>FACKTANGTAIPIGGGSANVYVNLAPVVNVGQNLVVDLSTQIFCHNDYPETITDYVTLQRGSAYGGVLSNFSGTVKYSGSSYPFPTTSETPRVVYNSRTDKPWPVALYLTPVSSAGGVAIKAGSLIAVLILRQ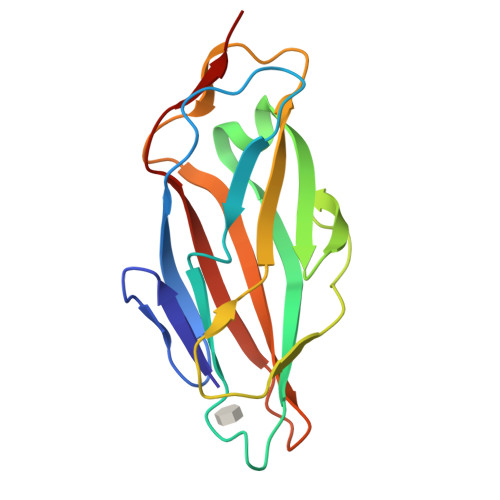TNNYNSDDFQFVWNIYANNDVVVPT[3x]> MSANDLPRGPEEGAPERKTREKPSQEQTDWSGSFSAYLESHRASLVDSLRRLFGHPFGSFFTCLVMGITLSLPMGLSLLLNNVERLGGSWQRAAQISLFLDLKTSENQGQDLREQIERLPDVIEAQLISREQALSELQEQSGLGEALKELPENPLPPVISVTPKQIDRAGLEALRQQLAELPHVQQAQLDLVWVERLSAILKLGERFVFGLTILLVLTLLLVVGNTIRLHIENRRNEIEVIKLVGGTDGYVRRPFLYMGALYGLGAGILSWALLAYSL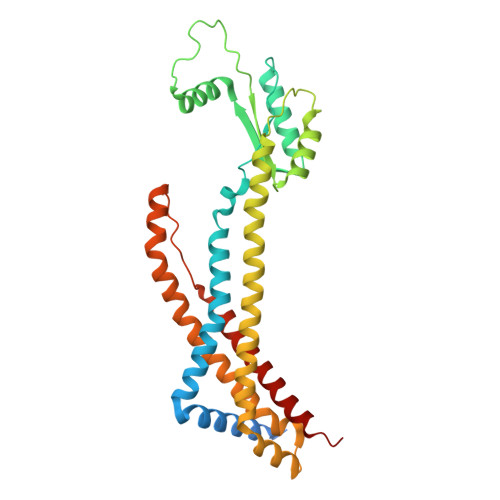NWLNGSVVNLSGLYGSDFGLQGVPLDDGLSLTVGAVLLGWVGAWLAVARHLRELAPR>[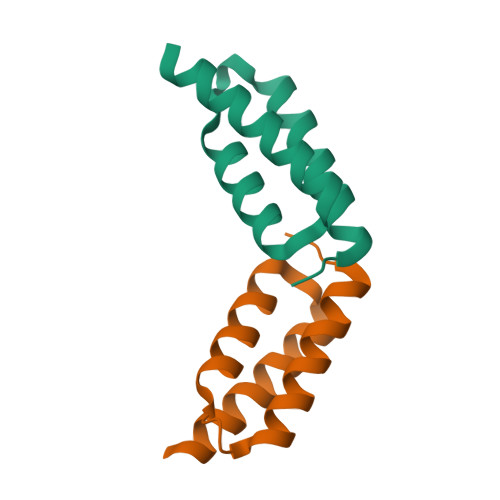2x]IKKEQKLIQAQNLVREFEKTHTVSAHRKAQKAVNLVSFEYKVKKMVLQERIDNVLKQGLVR>TELTKCKVSHAIKDIDGYQGISLLEWACVLFHTSGYDTQAVVNDNGSTEYGLFQISDRFWCKSSEFPESENICGISCDKLLDDELDDDIACAKKILAIKGIDYWKAYKPMCSEKLEQWRCEKP[2x];>[2x]ASMTGGQQMGRGSSLTACPEESPLLVGPMLIEFNIPVDLKLVEQQNPKVKLGGRYTPMDCISPHKVAIIIPFRNRQEHLKYWLYYLHPILQRQQLDYGIYVINQAGESMFNRAKLLNVGFKEALKDYDYNCFVFSDVDLIPMN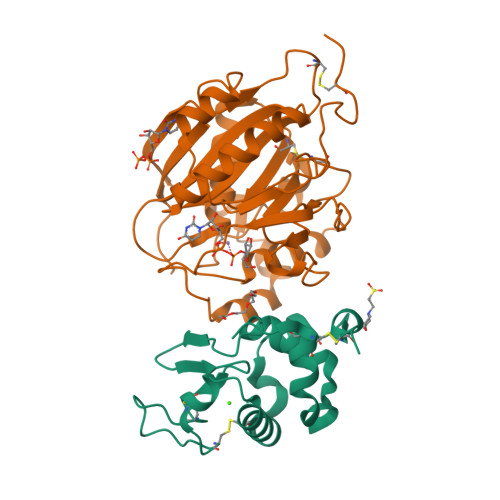DHNTYRCFSQPRHISVAMDKFGFSLPYVQYFGGVSALSKQQFLSINGFPNNYWGWGGEDDDIYNRLAFRGMSVSRPNAVIGKCRMIRHSRDKKNEPNPQRFDRIAHTKETMLSDGLNSLTYMVLEVQRYPLYTKITVDIGTPS>[4x]MAFKDLFKFNKGKTTFVFIGGKGGVGKTTISAATALWMARSGKKTLVISTDPAHSLSDSLEREIGHTPTKITENLYAVEIDPEVAMEEYQAKLQEQAAMNPGMGLDMLQDQMDMASMSPGIDEAAAFDQFLRYMTTDEYDIVIFDTAPTGHTLRLLSFPEIMDSWVGKMIKIRRQIGSMAKAFKNILPFMGDEEEEDRALQDMEATKKQINAAREVMSDPERTS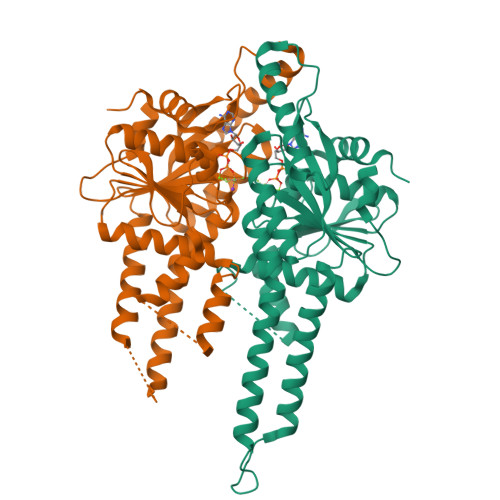FKMVVIPEEMSIYESERAMKALEKYSIHADGVIVNQVLPEESDCEFCNARRKLQQERLKQIREKFSDKVVAEVPLLKKEAKGIETLEKIAEQLYGEPEPE>[2x]SFMDRKEVVNIQTWINKPDIKHHFP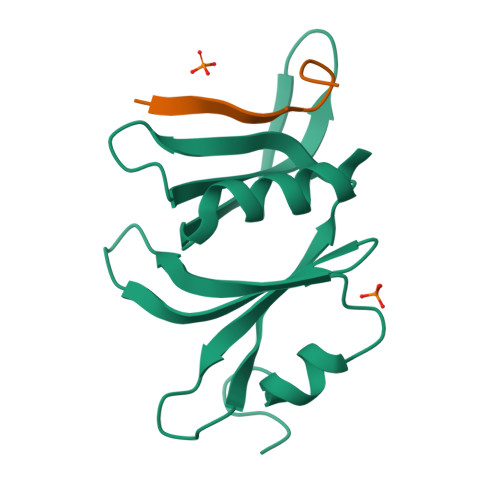CKEVKESGHMFPSHLLVTATHMYCLREILSRKGLAYIQSRQALNSVVKITSKKKHPELITFKYGNSSASGIEILAIERYLIPNAGDATRAIKQQIMK;>[2x]DDNTLYHRGFTED>[4x]MRGGALLCGQVQDEIEQLSRESSHFSLSTGILPSLGARSNRRVKLRR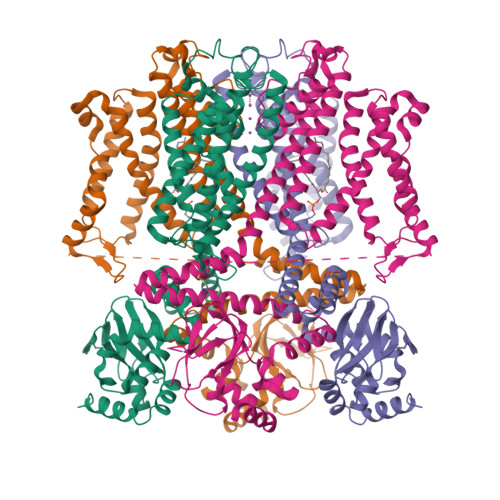FVVSPYDHKYRIWEAFLVVLVVYTAWVSPFEFGFLRKPRPPLSITDNIVNAFFAIDIIMTFFVGYLDKSTYLIVDDRKQIAFKYLRSWFLLDLVSTIPSEAAMRISSQSYGLFNMLRLWRLRRVGALFARLEKDRNFNYFWVRCAKLVCVTLFAVHCAACFYYLIAARNSNPAKTWIGANVANFLEESLWMRYVTSMYWSITTLTTVGYGDLHPVNTKEMIFDIFYMLFNLGLTAYLIGNMTNLVVHGTSRTRNFRDTIQAASNFAHRNHLPPRLQDQMLAHLCLKYRTDSEGLQQQETLDALPKAIRSSISHFLFYSLMDKVYLFRGVSNDLLFQLVSEMKAEYFPPKEDVILQNEAPTDFYILVNGTADLVDVDTGTESIVREVKAGDIIGEIGVLCYRPQLFTVRTKRLCQLLRMNRTTFLNIIQANVGDGTIIMNNLLQHLKEMNDPVMTNVLLEIENMLARGKMDLPLNLCFAAIREDDLLLHQLLKRGLDPNESDNNGRTPLHIAASKGTLNCVLLLLEYHADPNCRDAEGSVPLWEAMVEGHEKVVKVLLEHGSTIDAGDVGHFACTAAEQGNLKLLKEIVLHGGDVTRPRATGTSALHTAVCEENIEMVKYLLEQGADVNKQDMHGWTPRDLAEQQGHEDIKALFREKLHERRVHIETSSSVPILKTGIRFLGRFTSEPNIRPASREVSFRIRETRARRKTNNFDNSLFGILANQSVPKNGLATVDEGRTGNPVRVTISCAEKDDIAGKLVLLPGSFKELLELGSNKFGIVATKVMNKDNNAEIDDVDVIRDGDHLIFATDS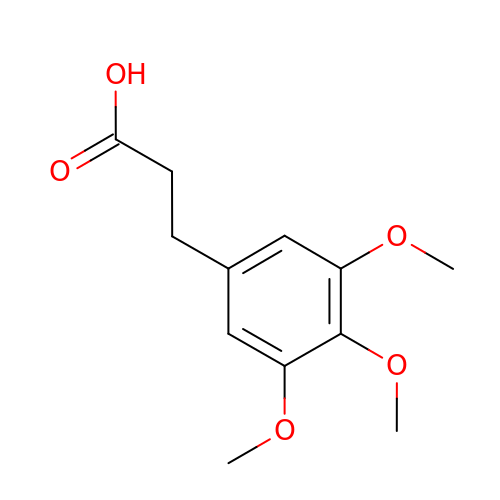3-(3,4,5-trimethoxyphenyl)propanoic acid | C12 H16 O5 | ZCYXGVJUZBKJAI-UHFFFAOYSA-N(R)-4-((4,4-dimethylpiperidin-1-yl)methyl)-2-hydroxy-N-((3-hydroxy-1-(6-((3-(methylcarbamoyl)benzyl)amino)pyrimidin-4-yl)piperidin-3-yl)methyl)benzamide 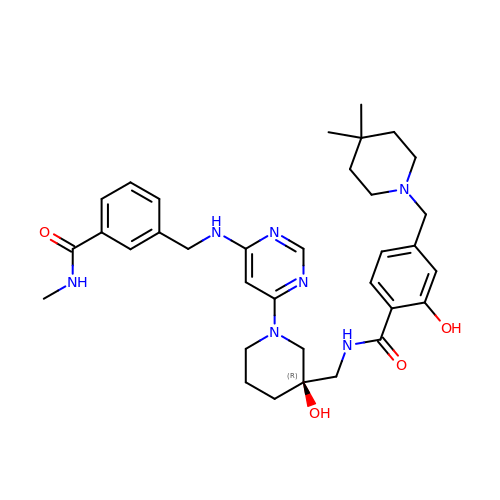| C34 H45 N7 O4 | HJSOUGSVWHGZMD-UUWRZZSWSA-N> PMEFEWDANKA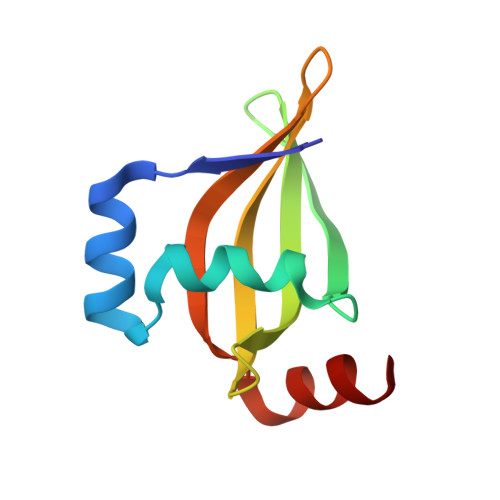KSNLRKHGVRFEDAVLVFDDPRHLSRQERYENGEYRWQTLGLVHGIVVILVAHSVRFESGFDVIRIISARKADRKERNRYEHG beta-D-xylofuranose | C5 H10 O5 | 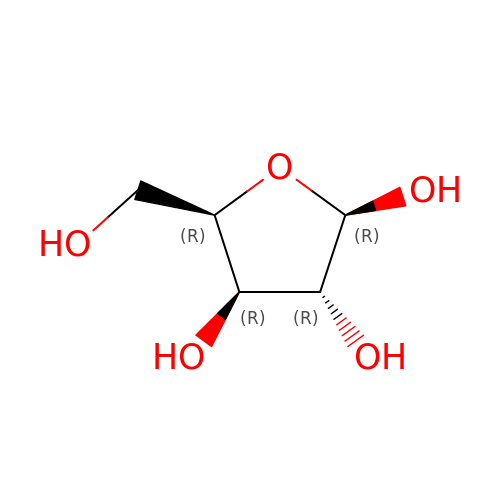HMFHBZSHGGEWLO-KKQCNMDGSA-N N-[2-(4-sulfamoylphenyl)ethyl]methanethioamide | C9 H12 N2 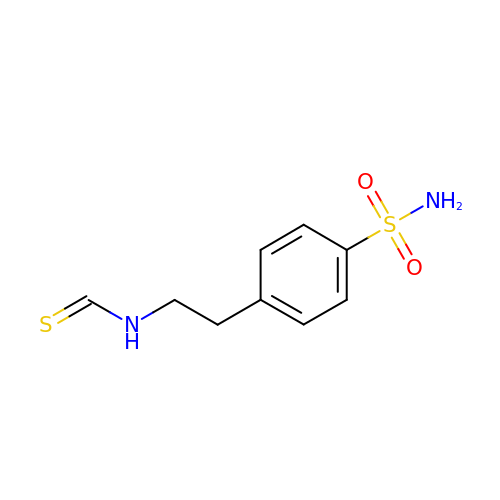O2 S2 | PXYIEGXZIBMDCF-UHFFFAOYSA-N>MSILSLTASQGQKATALANAVATATALLAVILFAVATRAASATKAEACQTPCQCSHQLRQAAAHYNSVLREAERKTDGHILQALKLLIAATGNNQKLQAAAVAPLATALKNWANCKAETGRLGTAARNNIDKLNAGAEAAAILANLTKLGGKVELTAKGGNGQLQQDSVTAEDLWRNTATECQIEEAEQGRHNFDPANSSDKMKLPKFNPVAKIGINCKKGGDTNNCNANAMAQNTGKLQFDVKIEAMGTQGGNDAASKWESAKAAEPVYITNELNIIAKTLESAGVANQALQNEFKQNSCA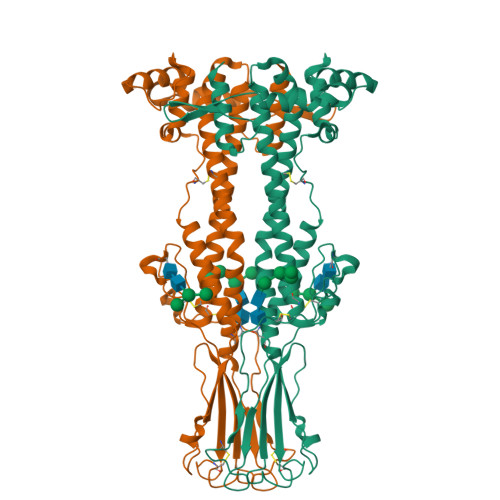EPSEEYSDFSNSGDFSRQIIRSYSNNKDNEKETTDKPSDLEKLIESAYGKNGAKFKENLWDQIDKLSPTVNKGETNEKLNLKTEKDISKLGEALARQLGYIRKEPEAAAEAQEKKTN[4x]>RHMQEILDAILSGDAASADYAALALPESYRAVTLHKGEERMFDGLASRDKDPRKSLHLDDVPLPELGPGEALVAVMASSVNYNTVWSSIFEPVSTFGFLERYGRLSPLTARHDLPYHVLGSDLAGVVLRTGAGVNAWKPGDEVVAHCLSVELESPDGHNDTMMDPEQRIWGFETNFGGLAQLALVKTNQLLPKPKHLTWEEAASPGLVNSTAYRQLVSRNGAGLKQGDNVLIWGASGGLGSYATQYALAGGATPICVVSSPRKADICRAMGAEAIIDRSAEGYRFWKDEHHQDPREWKRLGGKIREFTGGEDVDIVFEHPGRETFGASVYVTRKGGTIVTCASTSGYMHQYDN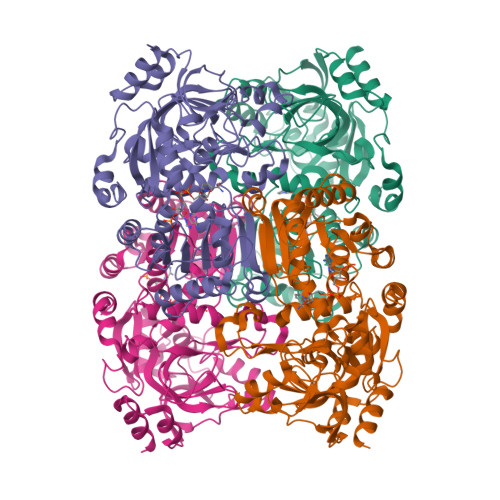RYLWMSLKRIVGSHFANYREAFEANRLVAKGKIHPTLSKVYALEETGQAALDVHHNKHQGKVGVLCLAPREGLGVTDPELRSKHLTKINAFR[4x]>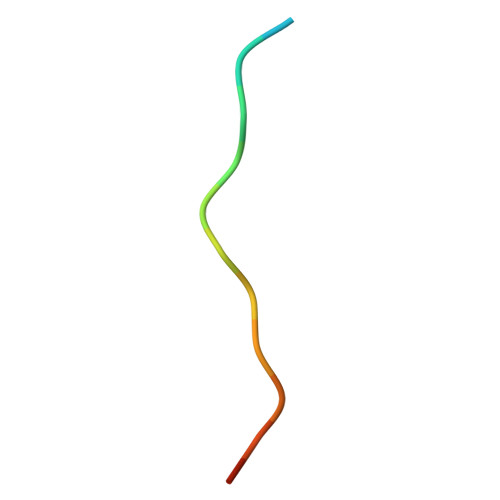 DDDDFGGFEAAETFD>[2x]LTLWTTLDPSPNCKIDIEKDSKLTLVLTKCGSQILANVSLIIVNGKFKILNNKTDPSLPKSFNIKLL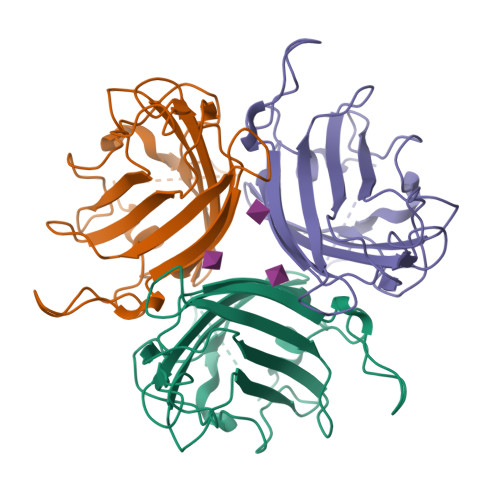FDQNGVLLENSNIEKQYLNFRSGDSILPEPYKNAIGFMPNLLAYAKATTDQSKIYARNTIYGNIYLDNQPYNPVVIKITFNNEADSAYSITFNYSWTKDYDNIPFDSTSFTFSYIAQE> MHTSVRWSETADAVKGIRPPVNSLCYSPSGDYVVASCGVRVLVYAASTGTLLHSLMGHQDTIYCVDYSSDGKNFASGGADRTVIVWSSQGEGIVKYQHTEAIQALAHNPTSSQLASVSSVDWGIWSPEQPKVSKYSLPSKGLCAAWTPNGKTLAIGMLDGTVMMLSKTSEEKVIIRRPAPVWALAFTPLRENGIDVLAIGSWDQRLSFYNLSGTAVGRERELDFDPCSVSYFNDGEYILLSGSDHKVTLFTKDGNRLIELASADDWIWSARQRPRQKQFCYGTNDGTISCIDITISTVHTIYDDQYVFRKDMTNLVVHQLLVDRKMVIPCNEYVQKIATFLDKLAVQLQERVIVFEFFYDDDRTMRYQDIAQIRRRLECSLLCVTTGAIIVSNDKRITMYDFQGNKRREWSMESPVQLMKVVGGMEGREILLVGLNGGQVMKVFVDNPFPTLLHKGTAPVKSAELSSSRSRLAVIDSTNTLQVLELGEKNELLFSEDNVTAVAFNIDVDDNIAFTTGDNTLHIKTGSLPAYQQAVRGIVVGFKANHVFNLHYSNMMVLDVPHAHALYKYVEMRDFDRAYEVACLGVADADWKMLGLHAMSQLRLDIARKAFTHIQDTKLVELLKSLELRRRQSGAEDGLSLTLGKASGTPDTVEGPENKGYGSTNGELAAARVAAKDSVLYGSILAFQGKYNDAARQFMKTGCELKAVEMYCDLKMWDNAKKICTDEKVLKDLIRQQARWAEESQNFVEAASLYESCGDYAKAIGMMGQAGQVEKLMKMCRSLPTSEVTLITECANFFRKHNAIPFAIEAYEKVQDHQALIGIYVAKGDWRNAFTILEKTPTLAREVYVPWATWLADNDKFDEALEAFRAAKWPKEAMRLMET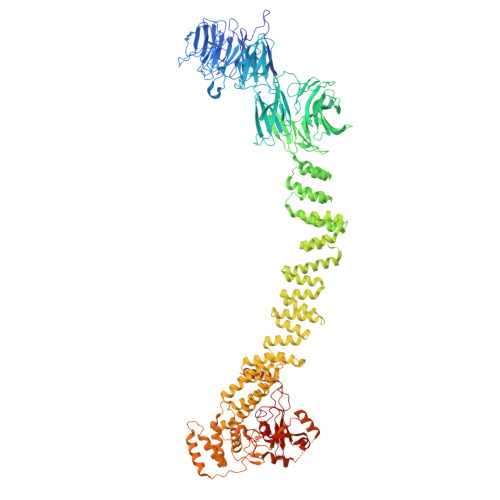LATNSVTCRKFRDAAFYYIHLAEEYGRFEETEKPTDVEKAARIRRSKECVRRADIYYAFSGVYAHTTQPLPYNELSLFRTAKYLFGMCAESAIPINVGKGAILYTLSRIANRLEMVRTARAVFEKLQGVILPVSMMEQVDIETLLVRSKPVKDRDELLDRCFRCNQLIAQLPMAGDRCPNCFHPCVRSFVNFECLPLVEFVLADELTDEEAERIIVSGVGRRRSADDENSKDHSDGADAKAKEWKSDNGANVISFDDGNIDYEIDQQLVAMGRSKAAANKGNDPFFTQLQYVLRPGRPTATYQPFVASADILKGFRRDEVFIVRPRYGTLPVPNRYYRLMRSDVSVCLCNGCQHFFIAEDYEAECMRGSGCPLCRYRPGKQVSRSMKQILFDMETAAAASKTSSAAAAL>[2x]MPERLQVYKCEVCGNIVEVLNGGIGELVCCNQDMKLMSENTVDAAKAKHVPVIEKIDGGYKVKVGAVAHPMEEKHYIQWIELLADDKCYTQFLKP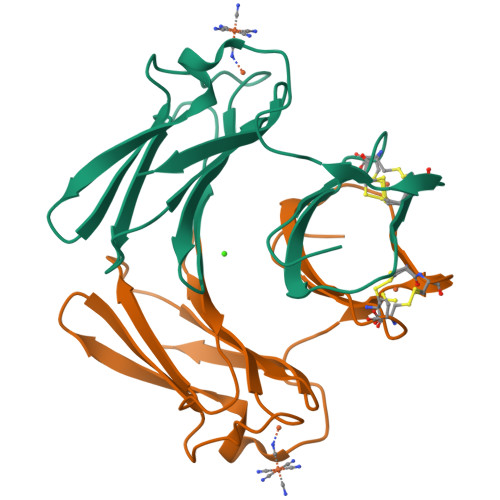GQAPEAVFLIEAAKVVAREYCNIHGHWKAEN> GG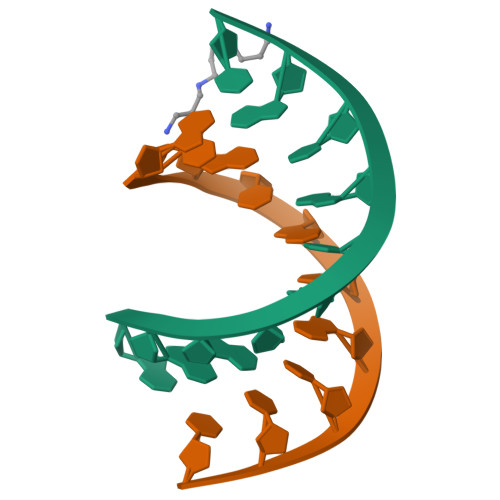GTATACGC;> GCGTATACCC PYRIDOXINE-5'-PHOSPHATE | C8 H12 N O6 P | 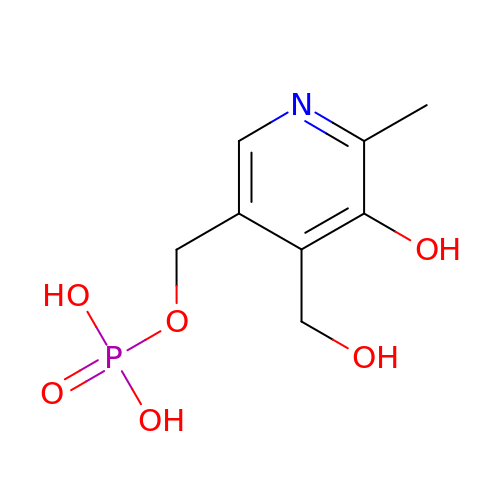WHOMFKWHIQZTHY-UHFFFAOYSA-N>MSFMDQIPGGGNYPKLPVECLPNFPIQPSLTFRGRNDSHKLKNFISEIMLNMSMISWPNDASRIVYCRRHLLNPAAQWANDFVQEQGILEITFDTFIQGLYQHFYKPPDINKIFNAITQLSEAKLGIERLNQRFRKIWDRMPPDFMTEKAAIMTYTRLLTKETYNIVRMHKPETLKDAMEEAYQTTALTERFFPGFELDADGDTIIGATTHLQ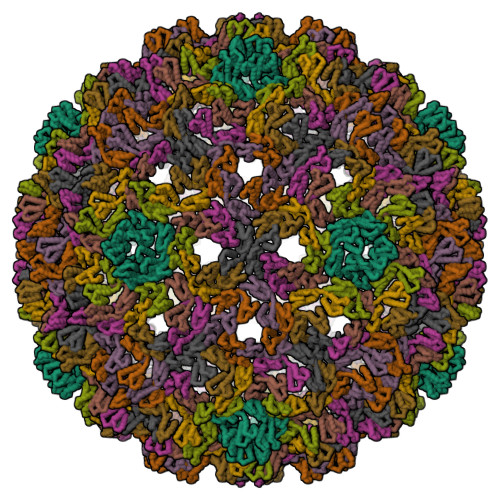EEYDSDYDSEDNLTQNRYVHTVRTRRSYNKPMSNHRNRRNNNASREECIKNRLCFYCKKEGHRLNECRARKAVLTDLELESKDQQTLFIKTLPIVH[9x]(2~{S})-2-methoxy-2-phenyl-~{N}-[5-[[(3~{R})-1-pyridazin-3-ylpyrrolidin-3-yl]amino]-1,3,4-thiadiazol-2-yl]ethanamide 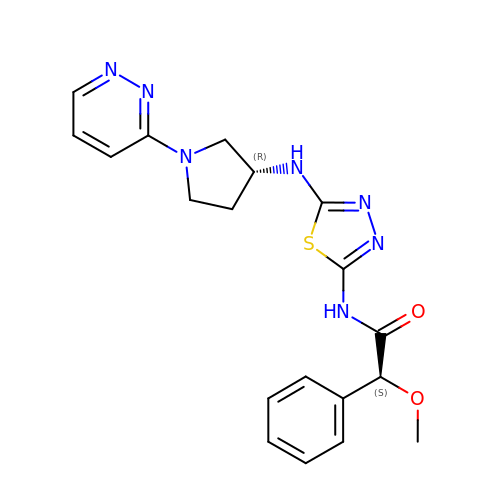| C19 H21 N7 O2 S | KLQLQDLJJUAEGT-ZBFHGGJFSA-N> V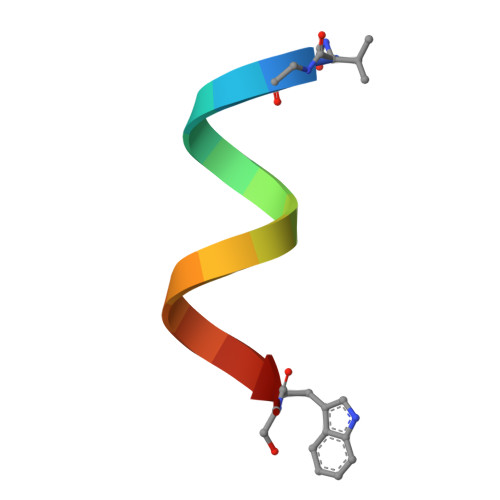GALAVVVWLWLWLWX> UUGCGUCGCGUCGAC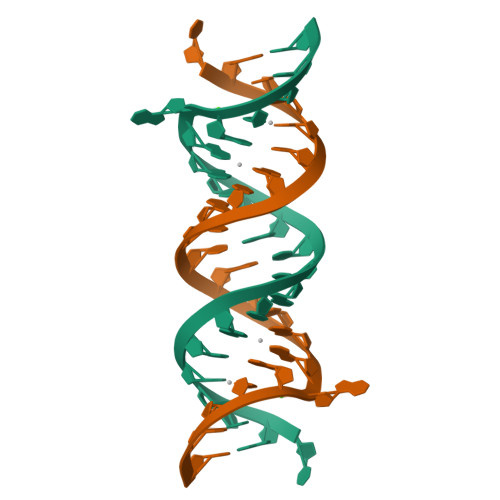GAAGUCGC> MTTQAPTFTQPLQSVVVLEGSTATFEAHISGFPVPE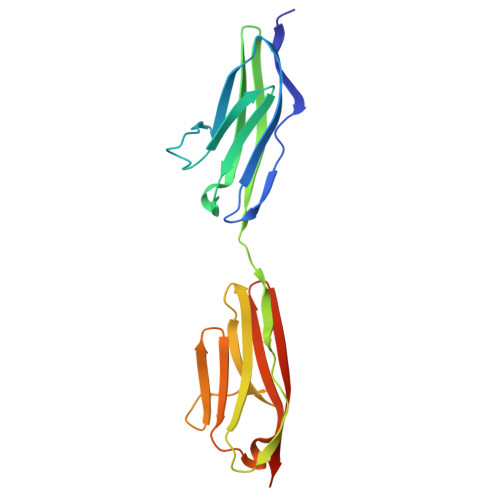VSWFRDGQVISTSTLPGVQISFSDGRAKLTIPAVTKANSGRYSLKATNGSGQATSTAELLVKAETAPPNFVQRLQSMTVRQGSQVRLQVRVTGIPTPVVKFYRDGAEIQSSLDFQISQEGDLYSLLIAEAYPEDSGTYSVNATNSVGRATSTAELLVQGETREEF> AFQETNPPAGPVRAIAEYERSAAVLVRYPFGIPMELIKELAKNDKVITIVASESQKNTVITQYTQSGVNLSNCDFIIAKTDSYWTRDYTGWFAMYDTNKVGLVDFIYNRPRPNDDEFPKYEAQYLGIEMFGMKLKQTGGNYMTDGYGSAVQSHIAYTENSSLSQAQVNQKMKDYLGITHHDVVQDPNGEYINHVDCWGKYLAPNKILIRKVPDNHPQHQ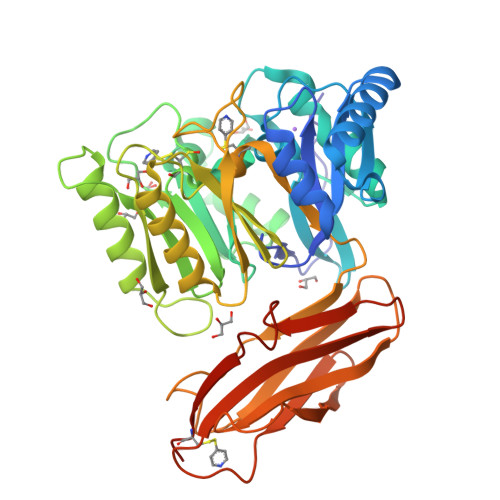ALEDMAAYFAAQTCAWGTKYEVYRALATNEQPYTNSLILNNRVFVPVNGPASVDNDALNVYKTAMPGYEIIGVKGASGTPWLGTDALHCRTHEVADKGYLYIKHYPILGEQAGPDYKIEADVVSCANATISPVQCYYRINGSGSFKAADMTMESTGHYTYSFTGLNKNDKVEYYISAADNSGRKETYPFIGEPDPFKFTCMNETNTCTVTGAA(TRANS-12,13-EPOXY)-9-HYDROXY-10(E)-OCTADECENOIC ACID | C18 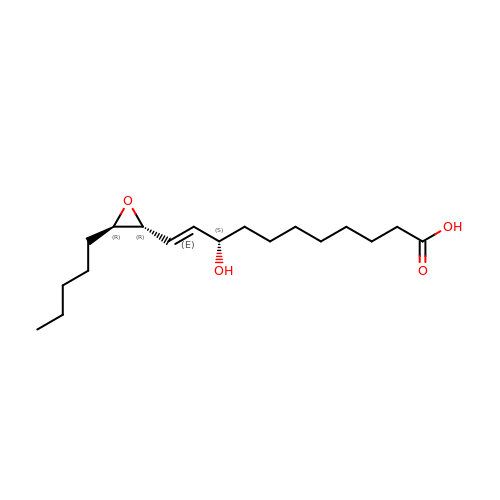H32 O4 | WCCLYKMJXGYGEN-WFZKJPOOSA-N> GSHMSNTQTVLPFT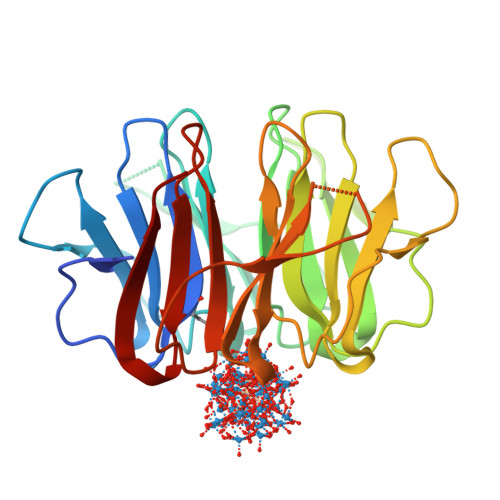GLNTPNGVAVDSAGTVYVTDKGNNRVVKLAAGSNTQTVLPFTGLNRPSGVAVDSAGTVWVTDHGNNRVVKLAAGSNTQTVLPFTGLNTPNGVAVDSAGTVYVTDKGNNRVVKLAAGSNTQTVLPFTGLNRPSGVAVDSAGTVWVTDHGNNRVVKLAAGSNTQTVLPFTGLNTPNGVAVDSAGTVYVTDKGNNRVVKLAAGSNTQTVLPFTGLNRPSGVAVDSAGTVWVTDHGNNRVVKLAAG>SNAMKTEKDKMLAGEMYIADDEELVADRVEAKRLTRLYNEAVETGDERRFTLLNQLLGSSADGKAQINPD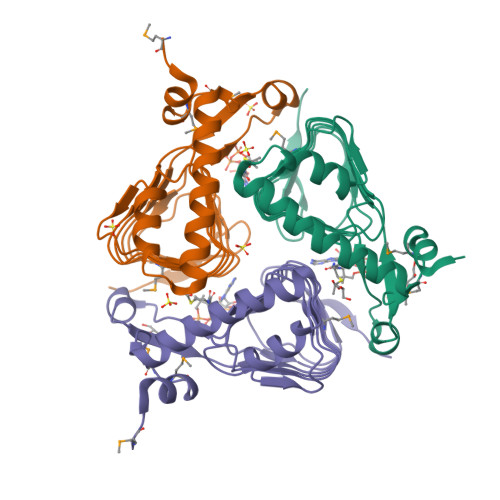FRCDYGYNIHVGKSFFANFNCVILDVCEVRIGDHCMFAPGVHIYTATHPLHPVERNSGKEYGKPVKIGNNVWVGGGAIINPGVSIGDNAVIASGAVVTKDVPNNVVVGGNPAKVIKTIEE[3x]>[2x]MMSIAQVRSAGSAGNFYTDKDNYYVLGSMGERWAGRGAEQLGLQGSVDKDVFTRLLEGRLPDGADLSRMQDGSNRHRPGYDLTFSAPKSVSMMAMLGGDKRLIDAHNQAVDFAVRQVEALASTRVMTDGQS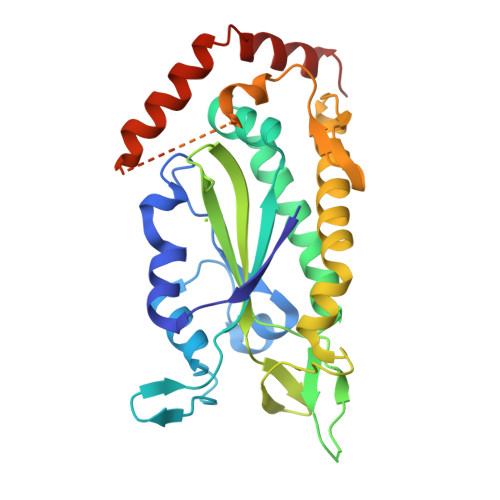ETVLTGNLVMALFNHDTSRDQEPQLHTHAVVANVTQHNGEWKTLSSDKVGKTGFIENVYANQIAFGRLYREKLKEQVEALGYETEVVGKHGMWEMPGVPVEAFSGRSQTIREAVGEDASLKSRDVAALDTRKSKQHVDPEIKMAEWMQTLKETGFDIRAYRDAADQRADS> SATRRYYLGAVELSWDYMQSDLGELPVDARFPPRVPKSFPFNTSVVYKKTLFVEFTDHLFNIAKPRPPWMGLLGPTIQAEVYDTVVITLKNMASHPVSLHAVGVSYWKASEGAEYDDQTSQREKEDDKVFPGGSHTYVWQVLKENGPMASDPLCLTYSYLSHVDLVKDLNSGLIGALLVCREGSLAKEKTQTLHKFILLFAVFDEGKSWHSETKNSLMQDRDAASARAWPKMHTVNGYVNRSLPGLIGCHRKSVYWHVIGMGTTPEVHSIFLEGHTFLVRNHRQASLEISPITFLTAQTLLMDLGQFLLFCHISSHQHDGMEAYVKVDSCPEEPQLRMKNNEEAEDYDDDLTDSEMDVVRFDDDNSPSFIQIRSVAKKHPKTWVHYIAAEEEDWDYAPLVLAPDDRSYKSQYLNNGPQRIGRKYKKVRFMAYTDETFKTREAIQHESGILGPLLYGEVGDTLLIIFKNQASRPYNIYPHGITDVRPLYSRRLPKGVKHLKDFPILPGEIFKYKWTVTVEDGPTKSDPRCLTRYYSSFVNMERDLASGLIGPLLICYKESVDQRGNQIMSDKRNVILFSVFDENRSWYLTENIQRFLPNPAGVQLEDPEFQASNIMHSINGYVFDSLQLSVCLHEVAYWYILSIGAQTD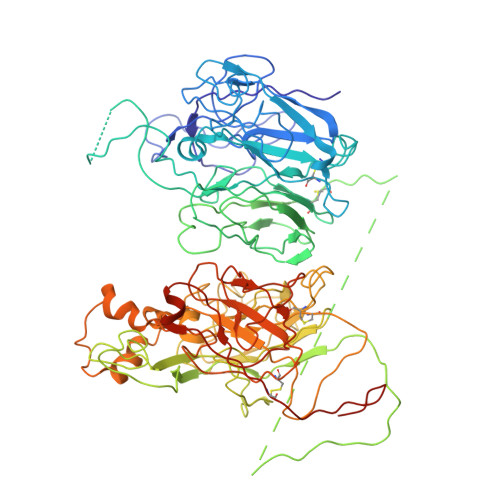FLSVFFSGYTFKHKMVYEDTLTLFPFSGETVFMSMENPGLWILGCHNSDFRNRGMTALLKVSSCDKNTGDYYEDSYEDISAYLLSKNNAIEPRS>SEELRAVADLQRLNIELARKLLEAVARLQELNIDLVRKTSELTDEKTIREEIRKVKEESKRIVEEAEEEIRRAKEESR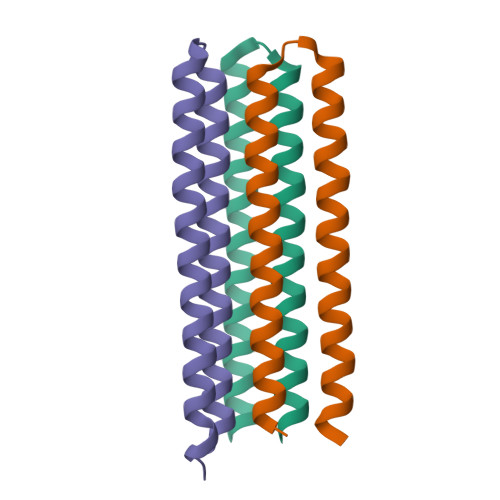YIADESRGSLEHHHHHH[6x]Among all SARS-CoV-2 encoded proteins, the nonstructural protein 3 (nsp3) is the largest, and it participates in many essential steps in the virus life cycle. In addition to the CoV-conserved domains of nsp3, SARS-CoV-2 nsp3 harbors a “SARS-Unique Domain” (SUD), which was first identified in the SARS-CoV genome. SUD contains three subdomains; there are two macrodomains, Mac2 and Mac3, that are followed by a frataxin-like Domain Preceding Ubl2 and PL2pro (DPUP). SUD-core does not possess enzymatic activity; rather, it functions as a binding module for viral and host molecules.

Therefore, we engineered a disulfide bond in SARS-CoV-2 SUD-core based on SARS-CoV SUD-core; the resulting mutant containing double mutations L516C-Y647C was denoted SARS-CoV-2 SUD-core-CC. The crystals of SARS-CoV-2 SUD-core-CC belonged to the space group of P321 and the best crystals diffracted the X rays to 1.35 Å resolution. After the screening of SUD-binding compounds (detailed in bellow sections), the SUD crystals co-crystallized with the hit compound 4 diffracted to the highest resolution 1.35 Å, thus was used for in depth analysis. Our highest-resolution dataset (1.35 Å resolution) was obtained by co-crystalizing SARS-CoV-2 SUD-core-CC with Comp.4, suggesting that it interacted with SUD during crystallization. However, the electron density of TF3 could not be located. SUD-core-CC comprises tandem SUD-N and SUD-M macrodomains connected by a flexible loop region. A nine-residue loop region between SUD-N and SUD-M (residues 541-549) is completely missing from the electron density map despite its atomic resolution, suggesting that this interdomain linkage is highly flexible. We clearly observed the engineered disulfide bond between L561C and Y647C, tethering SUD-N and SUD-M together. We superimposed SARS-CoV-2 SUD-core-CC and SARS-CoV SUD-core, and 257 Cα atoms aligned with a Dali Z-score of 24.1, and a root mean square deviation (RMSD) of 2.6 Å. This high structural deviation stemmed from distinct interdomain orientations between SUD-N and SUD-M in the two SUD structures, rather than differences in the individual domains themselves.

> KIKACVEEVTTTLEETKFLTENLLLYIDINGNLHPDSATLVSDIDITFLKKDAPYIVGDVVQEGVLTAVVIPTKKAGGTTEMLAKALRKVPTDNYITTYPGQGCNGYTVEEAKTVLKKCKSAFYILPSIISNEKQEILGTVSWNLREMLAHAEETRKLMPVCVETKAIVSTIQRKYKGIKIQEGVVDYGARFYFYTSKTTVASLINTLNDLNETLVTMPLGYVTHGLNLEEAARCMRSLKVPATVSVSSPDAVTAYNGYLTSSS> TLSILVAHDLQRVIGFENQLPWHLPNDLKHVKKLSTGHTLVMGRKTFESIGKPLPNRRNVVLTSDTSFNVEGVDVIHSIEDIYQLPGHVFIFGGQTLFEEMIDKVDDMYITV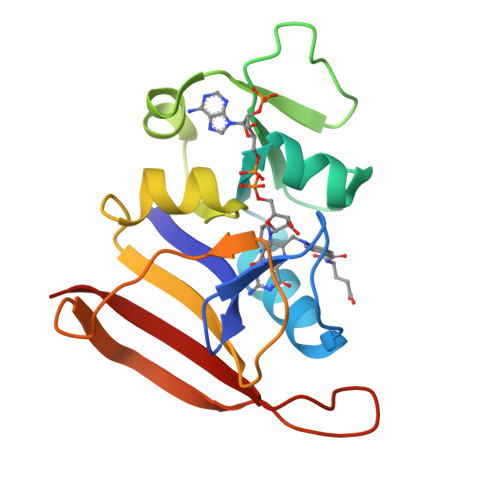IEGKFRGDTFFPPYTFEDWEVASSVEGKLDEKNTIPHTFLHLIRKK> SFRIEYDTFGELKVPNDKYYGAQTVRSTMNFKIGGVTERMPTPVIKAFGILKRAAAEVNQDYGLDPKIANAIMKAADEVAEGKLNDHFPLVVWQTGSGTQTNMNVNEVISNRAIEMLGGELGSKIPVHPNDHVNKSQSSNDTFPTAMHIAAAIEVHEVLLPGLQKLHDALDAKSKEFAQIIKIGRTHTQDAVPLTLGQEFSGYVQQVKYAMTRIKAAMPRIYELAAGGTAVGTGLNTRIGFAEKVAAKVAALTGLPFVTAPNKFEALAAHDALVELSGAMNTTACSLMKIANDIRFLGSGPRSGLGELILPENEPGSSIMPGKVNPTQCEAMTMVAAQVMGNHVAVTVGGSNGHFELNVFKPMMIKNVLHSARLLGDASVSFTENCVVGIQANTERINKLMNESLMLVTALNPHIGYDKAAKIAKTAHKNGSTLKE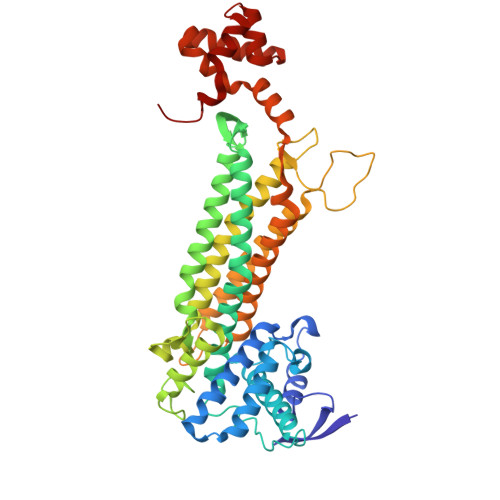TAIELGYLTAEQFDEWVKPKDMLGPK>EEIMRDDNMMFITKKMIEIRNLLQKVGQGSTVTLPSIVVIGSQSSGKSSVLEAIVGHEFLPKGSNMITRRPIELTLVNDPEAKVDYGEFPDLGLARVTDFSLIQKTLTELNQSVPESECVTDDPIRLTIHSPNIPDLSLIDLPGYIQVAGENQPRELKRKITELCDKYIRGPNIILAISAADTDLANSTALQASRRVDPRGERTIGVITKMDLVEPEKGAAILSDRQYPLKLGYVGVISKLPPQSGLFRRDTGNLLASINRNEKNYFGSHPTEFGPDSGVSTGVMTLRKKLLQVLEQQMSSKLNETTEAIQRELEETTYQFKVQYNEQPMSAESYLAASLDDFKHQFHEFASSFGRPQLQTLLKDALDQKVLDQLAARYWNRPIEDLSPAPREPDNIIDLPKADPDSPYWHRQLDTACSGLTRLGVGRLAATVAASAIQQHVEKLLDKSSFAKHPSARKVISDAAATVLADRSYATSDGIEISLKPYKFDPDIQPNEWAQGREHVVGVLQAELEQCQAAMKALENSVGGRKKLKEVMSFVDKARKGEIIVEGDHPSGAGGFSAALLARGREAVFLRDRADILSLRIQAAKSRQCKTLTNKYYCPEVFLDAVATKLAQTAVLFLNVEMLNDFYVRFPREVEAKLHEHMHAGGGLEKFAREDPKVRRHLDL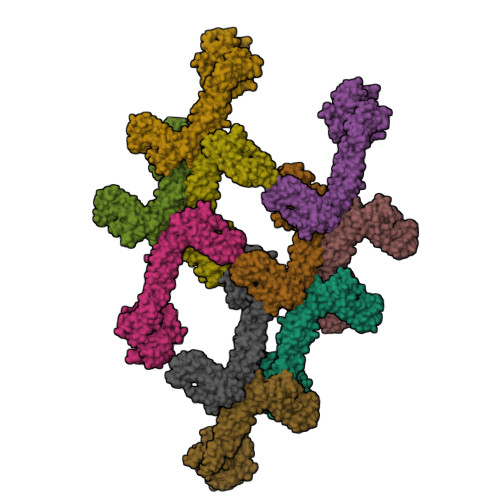IRRKELLETVLGKIEELHRISSGTAG[10x]>HP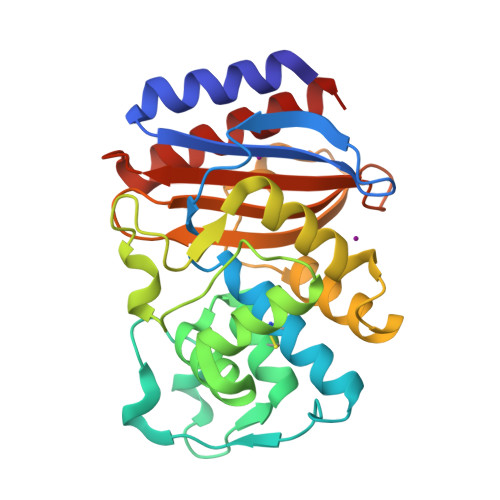ETLVKVKDAEDQLGARVGYIELDLNSGKILESFRPEERFPMMSTFKVLLCGAVLSRVDAGQEQLGRRIHYSQNDLVEYSPVTEKHLTDGMTVRELCSAAITMSDNTAANLLLTTIGGPKELTAFLHNMGDHVTRLDRWEPELNEAIPNDERDTTTPAAMATTLRKLLTGELLTLASRQQLIDWMEADKVAGPLLRSALPAGWFIADKSGAGERGSRGIIAALGPDGKPSRIVVLYTTGSQATMDERNRQIAEIGASLIKHW[4x]> MHNHNHNHNHNHNGGENLYFQGASLTEIEHLVQSVCKSYRETCQLRLEDLLRQRSNIFSREEVTGYQRKSMWEMWERCAHHLTEAIQYVVEFAKRLSGFMELCQNDQIVLLKAGAMEVVLVRMCRAYNADNRTVFFEGKYGGMELFRALGCSELISSIFDFSHSLSALHFSEDEIALYTALVLINAHRPGLQE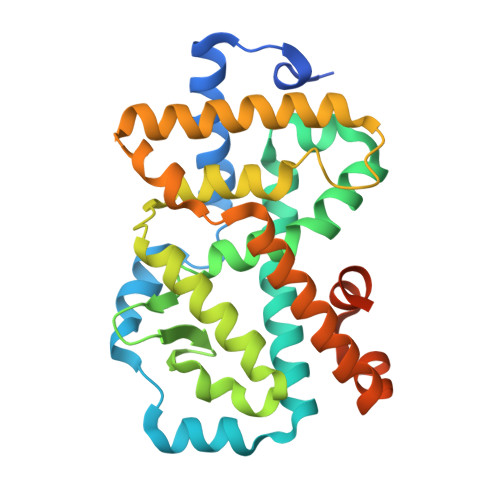KRKVEQLQYNLELAFHHHLCKTHRQSILAKLPPKGKLRSLCSQHVERLQIFQHLHPIVVQAAFPPLYKELFSGGSGGSGGKEKHKILHRLLQDSS> XEDIIRNIARHLALVGDLLDRS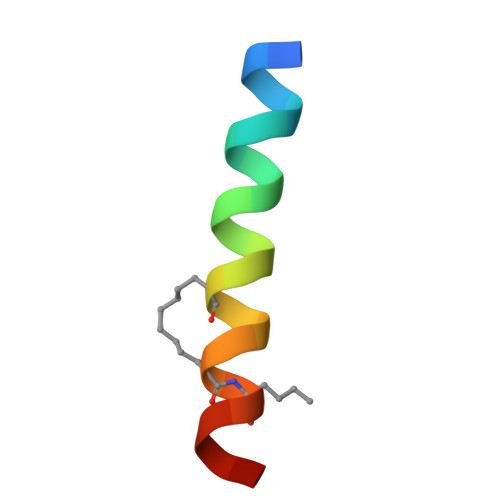IW>[3x]SNAMNQEFFMLSQAMVEHLNEQINLEFFSSNLYLQMSAWCEDKGFDGAAEFLRAHAVEEMQHMQRLFTYVSETGALPILGAIAA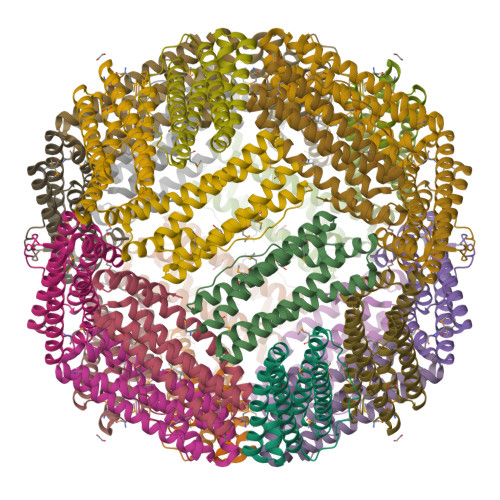PRHDFASLGEVFRETYQHEQKITQQINKLAHVAFTSQDYSTFNFLQWYVAEQHEEEKLFKGILDKLELVGEDGKALFFIDKDLAALAKKGSSSVMDAPAE>[6x]MIVPVLSRQALRHASVARVALPSLTRWYASYPPHTVVKMPALSPTMTSGGIGAWQKKPGDKIEPGEVLVEIETDKAQMDFEFQEEGVLAKILKDSGEKDVAVGNPIAILVEEGTDVNAFKDFTLKDAGGETSPAVPKDEPKNESTASAPTPAPTPAPEPENTSFTGRFQTALEREPNALPAAKRLAREKGIDLRNVKGSGPGGKITEEDVKKALASAPAAGAAAAAYTDVPISGMRKTIAARLKESVTENPHFFVSTNLSVSKLLKLRQALNSSADGRYKLSVNDFLIKAMGIASKRVPTVNSSWRDGVIRQFETVDVSVAVATPNGLITPIVKGVEGKGLESISAAVKELAKKARDGKLKPEEYQGGSISISNMGMNPAVQSFTAIINPPQAAILAVGAPQKVAVPVENEDGTTGVSWDEQIIVTASFDHKVVDGAVGAEWIRELKKVIENPLELLL;>MASLTAACRISARMAGRSVRGFRT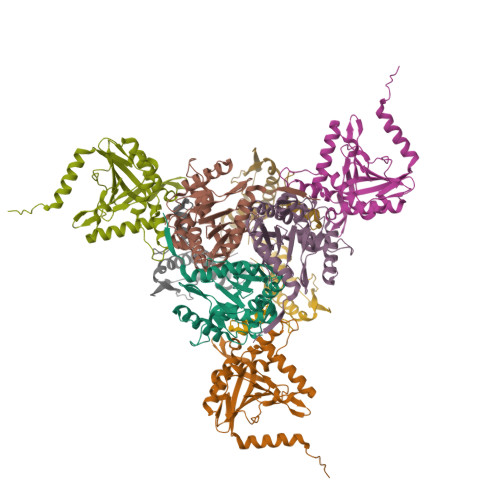SAAALAAQNFTMPALSPTMTEGNIATWRVKEGDKFSAGDVLLEIETDKATMDVEAQDDGVMVKIMKNDGAKGVAVGARIAVIAEEGDDISSLEIPADAAPQSKPAESAPSAPPPPTTADQSNVAVPESAPQNASSKSAPKPPKRQYPHYPSVAHLLKVNGIDAAAVKDITPTGPGGRLLKGDVLAYLGKINAQTPSTVSERFEKQSHLDLSNIKVAKSTEAVKATTEKAQSKKLDAPAPPPVAVVTAPISLSAAIDVQNKLHKTIGVFLPLSTFITRATEIANQKLPLPANYQPTADELFNQVLGLDKVTRKESRGSYTPTFGSFVAPQRAARKADIIDILAAPSTRVAASAQSKSAAPGLTTSGPNVFSLQVPKSEEKRAQAFLQKMKLVLEQEPDKLVRA[3x]>DRHHHHHHKLQHAPPWTEDCRKSTYPPSGPTYRGAVPWYTINLDLPPYKRWHELMLDKAPMLKVIVNSLKNMINTFVPSGKVMQVVDEKLPGLLGNFPGPFEEEMKGIAAVTDIPLGEIISFNIFYELF[2x];>[2x]TICTSIVAEDKKGHLIHGRNMDFGVFLGWNINNDTWVITEQLKPLTVNLDFQRNNKTVFKASSFAGYVGMLTGFKPGLFSLTLNERFSINGGYLGILEWILGKKDAMWIGFLTRTVLENSTSYEEAKNLLTKTKILAPAYFILGGNQSGEGCVITRDRKESLDVYELDAKQGRWYVVQTNYDRWKHPFFLDDRRTPAKMCLNRTSQENISFETMYDVLSTKPVLNKLTVYTTLIDVTKGQF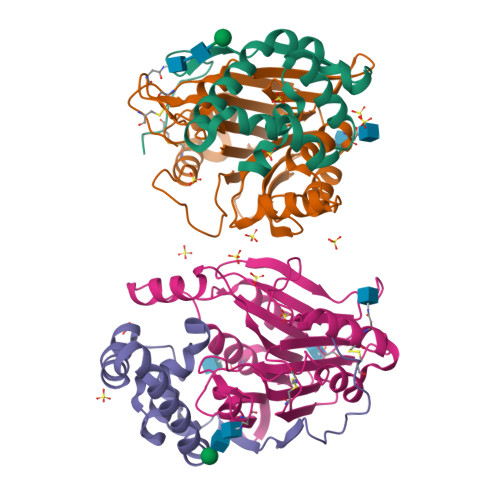ETYLRDCPDPCIGW>[2x]NYPAEPFRIKSVETVSMIPRDERLKKMQEAGYNTFLLNSKDIYIDLLTDSGTNAMSDKQWAGMMMGDEAY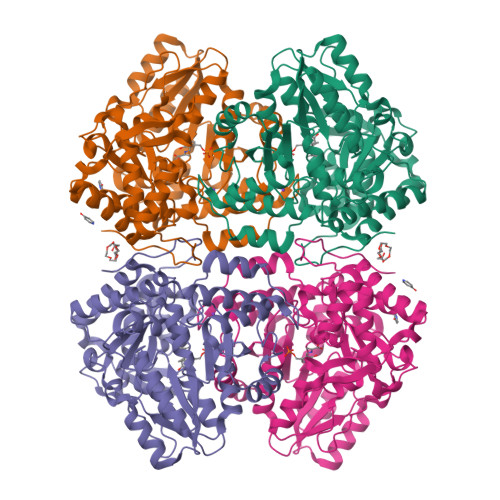AGSENFYHLERTVQELFGFKHIVPTHQGRGAENLLSQLAIKPGQYVAGNMYFTTTRYHQEKNGAVFVDIVRDEAHDAGLNIAFKGDIDLKKLQKLIDEKGAENIAYICLAVTVNLAGGQPVSMANMRAVRELTAAHGIKVFYDATRCVENAYFIKEQEQGFENKSIAEIVHEMFSYADGCTMSGKKDCLVNIGGFLCMNDDEMFSSAKELVVVYEGMPSYGGLAGRDMEAMAIGLREAMQYEYIEHRVKQVRYLGDKLKAAGVPIVEPVGGHAVFLDARRFCEHLTQDEFPAQSLAASIYVETGVRSMERGIISAGRNNVTGEHHRPKLETVRLTIPRRVYTYAHMDVVADGIIKLYQHKEDIRGLKFIYEPKQLRAFTARFDYI> APAVADKADNAFMMICTALVLFMTIPGIALFYGGLIRGKNVLSMLTQVTVTFALVCILWVVYGYSLAFGEGNNFFGNINWLMLKNIELTAVMGSIYQYIHVAFQGSFACITVGLIVGALAERIRFSAVLIFVVVW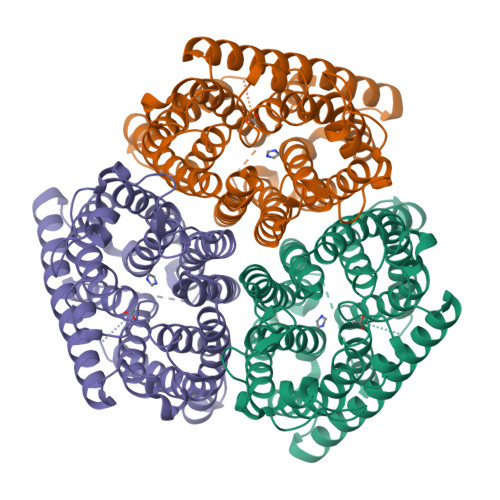LTLSYIPIAHMVWGGGLLASHGALDFAGGTVVFINAAIAGLVGAYLIGKRVGFGKEAFKPHNLPMVFTGTAILYIGWFGFNAGSAGTANEIAALAFVNTVVATAAAILGWIFGEWALRGKPSLLGACSGAIAGLVGVTPACGYIGVGGALIIGVVAGLAGLWGVTMLKRLLRVDDPCDVFGVHGVCGIVGCIMTGIFAASSLGGVGFAEGVTMGHQLLVQLESIAITIVWSGVVAFIGYKLADLTVGLRVPEEQEREGLDVNSHGENAYNADQAQQPAQADLEHHHHHH>[6x]MFEIKKICCIGAGYVGGPTCSVIAHM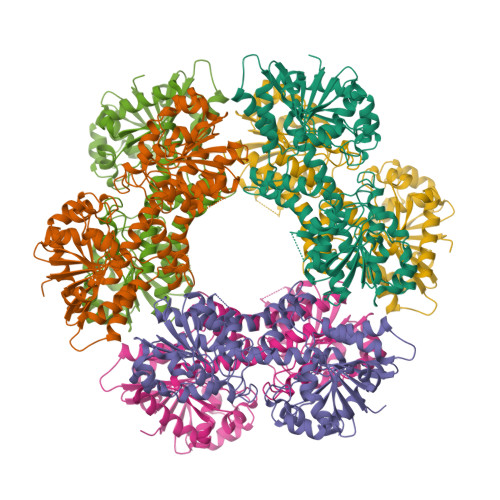CPEIRVTVVDVNESRINAWNSPTLPIYEPGLKEVVESCRGKNLFFSTNIDDAIKEADLVFISVNTPTKTYGMGKGRAADLKYIEACARRIVQNSNGYKIVTEKSTVPVRAAESIRRIFDANTKPNLNLQVLSNPEFLAEGTAIKDLKNPDRVLIGGDETPEGQRAVQALCAVYEHWVPREKILTTNTWSSELSKLAANAFLAQRISSINSISALCEATGADVEEVATAIGMDQRIGNKFLKASVGFGGSCFQKDVLNLVYLCEALNLPEVARYWQQVIDMNDYQRRRFASRIIDSLFNTVTDKKIAILGFAFKKDTGDTRESSSIYISKYLMDEGAHLHIYDPKVPREQIVVDLSHPGVSEDDQVSRLVTISKDPYEACDGAHAVVICTEWDMFKELDYERIHKKMLKPAFIFDGRRVLDGLHNELQTIGFQIETIGKKVSSKRIPYAPSGEIPKFSLQDPPNKKPKV>SHMENSGGNAFVPAGNQQEAHWTINLKDADIREFIDQISEITGETFVVDPRVKGQVSVVSKAQLSLSEVYQLFLSVMSTHGFTVVAQGDQARIVPNAEAKTEAGGGQSAPDRLETRVIQVQQSPVSELIPLIRPLVPQYGHLAAVPSANALIISDRSANIARIEDVIRQLDQKGSHDYSVINLRYGWVMDAAEVLNNAMSRGQAKGAAGAQVIADARTNRLI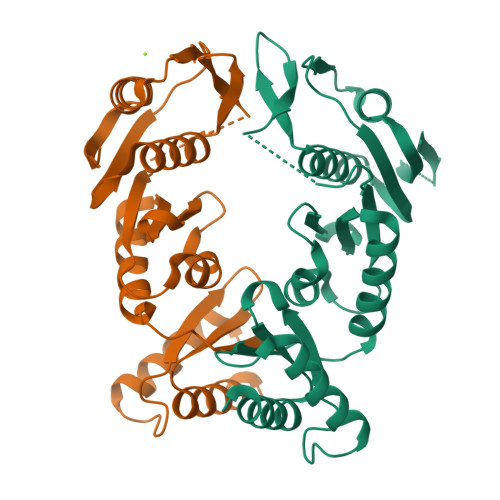ILGPPQARAKLVQLAQSLDTPTAR[2x]>GSFTSTSLSDQKYLSSSSSSSSNADPNKRIF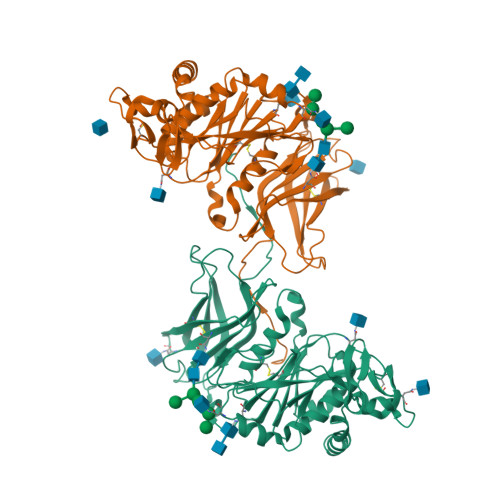QAYGNAAALFVQMGAYRGGPTTFAVVGLASKPIHVFRLPWYKCEWISNNGSSIRAKAYKMLPDWGYGRVYTVVVVNCTFPVNPNQDNAGGRLMLNAYYDESQRKYEKFTALEELPGSYNESKFRPPYQYEYLYCGSSLYGNLSASRFREWMAYHAWFFGPSSHFVFHDAGGVSPEVRAALDPWVRAGRATVQDIRGQAEFDGYYYNQFLVVNDCLHRYRYSANWTFYFDVDEYIYLPEGNTLESVLKDFSNYTQFTIEQNPMSSALCFNDSTQDYPRQWGFEKLLFRESRTGIRRDRKYAIQAKNAYATGVHMSENVIGKTLHQTETKIRYYHYHNSIQVPGELCREFLPLSAKNNVTWYNGLPYVYDDNMKKLASTIKDFERNTIGNVQAYS[4x]> MSIVNILSVNVLNNPAKFSDPYKFEITFECLEPLKSDLEWKLTYVGSATSQSYDQILDTLLVGPIPIGINKFVFEADPPNIDLLPQLSDVLGVTVILLSCAYEDNEFVRVGYYVNNEMEGLNLQEMDDAEI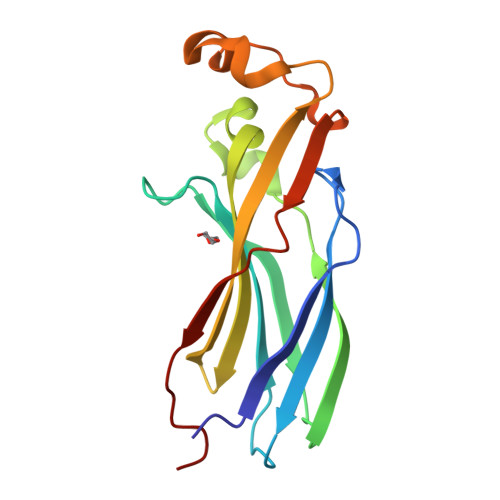KKVKVDISKVWRSILAEKPRVTRFNIQWDN> DEITKKYIKDNIINVDDNIIKKKDIFKLKNENNEITECAFEYFESKKKFDDDIESRFFIINDNNYNENINLIYKDIKYCGLNIQTTGLEVFDENIRLIQIAVENYPVIIYDMFNINKKDILDGLRKVLENKNIIKIIQNGKFDAKFLLHNNFKIENIFDTYIASKLLDKNKNMYGFKLNNIVEKYLNVILDKQQQNSVWNNSLLNNNQLFYAARDSSCLLKLYKKLKEEIKKENLHIVNDIENKCILPICDMELNGIKVDLENLQKSTNEILNELNIEKDNLKKKLKDENINVNSQQQVLKALQKNNVRDISNKLIENTSDSNLKNFLNHEEIISLRNYRRLYKLYSAFYLKLPLHINTKTNKIHTTFNQLKTFSGRFSSEKPNLQQIPRQKNIREIFIPNDNNIFIIADFKQIELKIAAEITNDEIMLKAYNNNIDLHTLTASIITKKNIPDINKEDRHIAKAINFGLIYGMNYVNLKNYANTYYGLNMSLDQCLYFYNSFFEHYKGIYKWHNQVKQKRALQYSTLSNRKVIFPYFSFTKALNYPVQGTCADILKLALVDLYDNL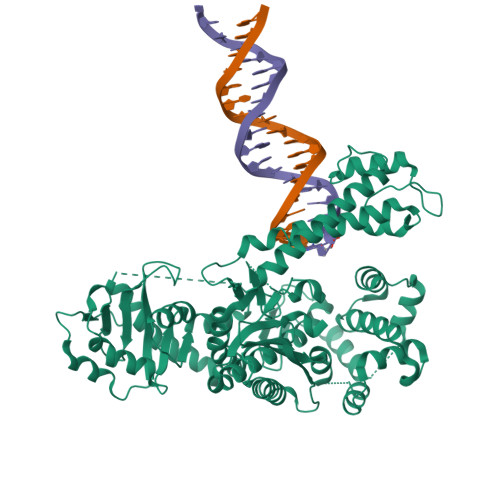KDINGKIILCVHDEIIIEVNKKFQEEALKILVQSMENSASYFLKKVKCEVSVKIAENWGSKD(~{E})-3-[4-oxidanyl-3-(5-prop-2-enyl-2-propoxy-phenyl)phenyl]prop-2-enoic 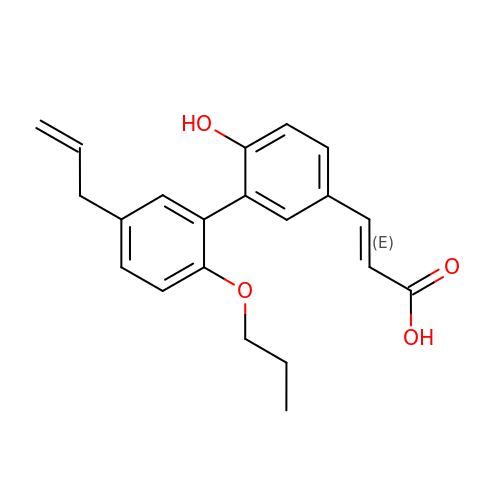acid | C21 H22 O4 | UZQZYUBWKWMBDW-DHZHZOJOSA-N>[4x]MKILVASRNPKKLAELSRVLESSGVSGVELVSLTDVPEYEEVPETG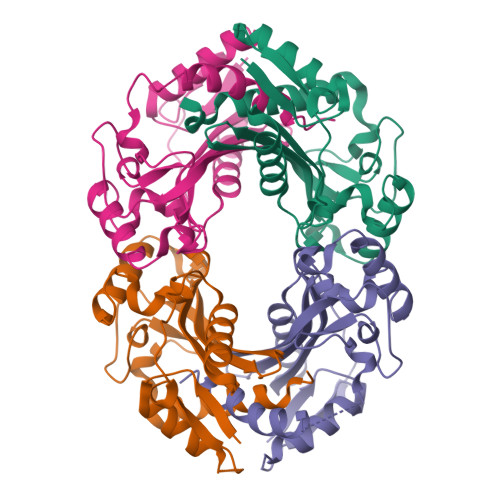ASFEDNALIKAREGVKHTGLACVADDSGLAVDALNWMPGVLSARWSGRHGDDAANTALLLAQLSDIPDERRGAAFVSACALVTPEGEEVVVEGRWKGSIARIPAGQNGFGYDPIFVPRGGLRTAAELTPEEKDAVSHRGRALAALLPMLRNLVNLGRTAPGHHHHHH> MSLQYGAEETPLAGSYGAADSFPKDFGYGVEEEEEEAAAAGGGVGAGAGGGCGPGGADSSKPRILLMGLRRSGKSSIQKVVFHKMSPNENLFLESTNKIYKDDISNSSFVNFQIWDFPGQMDFFDPTFDYEMIFRGTGALIYVIDAQDDYMEALTRLHITVSKAYKVNPDMNFEVFIHKVDGLSDDHKIETQRDIHQRANDDLADAGLEKLHLSFYLTSIYDHSIFEAFSKVVQKLIPQLPTLENLLNIFISNSGIEKAFLFDVVSKIYIATDSSPVDMQSY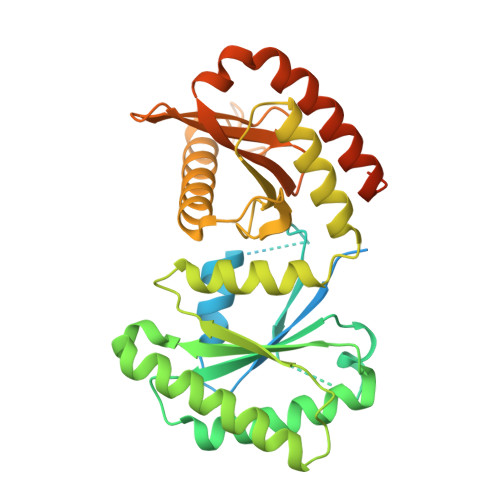ELCCDMIDVVIDVSCIYGLKEDGSGSAYDKESMAIIKLNNTTVLYLKEVTKFLALVCILREESFERKGLIDYNFHCFRKAIHEVFEVGVTSHRSCGHQTSASSLKALTHNGTPRNAI> GSKPMEVYVSAVASPTKFWVQLIGPQSKKLAS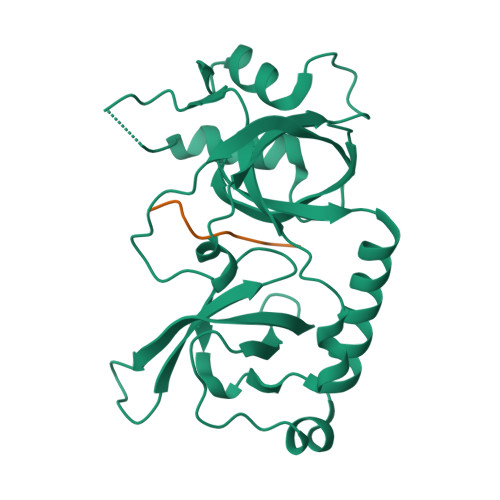MVQEMTSYYSSAENRAKHVLTAPYVGQIVAAVFKFDEKWYRAEIVDIMPNQYNPKEQVIDLYFVDYGDSEYISPADICELRTDFLTLRFQAVECFLANVKSTIQTEPITWPKSSIAKFEELTEVAHWRKLIARVVTYKERPRATTAVSAAAKEGTPLPGVELFDPADNSELNIADLMITQGFALPLDDSYP;> DQGRGRRRP> ANPLYQKHIISINDLSRDDLNLVLATAAKLKANPQPELLKHKVIASAFFEASTRTRLSFETSMHRLGASVVGFSD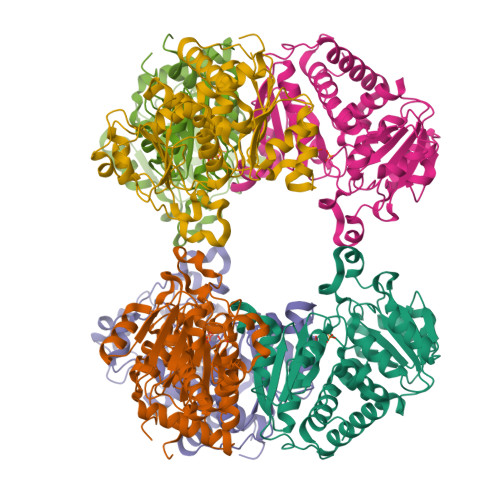SANTSLGKKGETLADTISVISTYVDAIVMRHPQEGAARLATEFSGNVPVLNAGDGSNQHPTQTLLDLFTIQETQGRLDNLHVAMVGDLKYGRTVHSLTQALAKFDGNRFYFIAPDALAMPQYILDMLDEKGIAWSLHSSIEEVMAEVDILYMTRVQKERLDPSEYCNVKAQFVLRASDLHNAKANMKVLHPLPRVDEIATDVDKTPHAWYFQQAGNGIFARQALLALVLNRDLVL> MTNTDLKPLLDNLRNATEF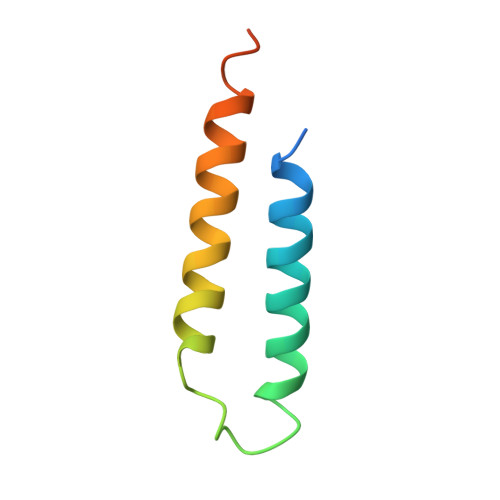WNLVKEASATDESTVHNRSYRDALDWLESAALALGDALIAQRKAVGGDHE4-(3-carboxyphenyl)pyridine-2,5-dicarboxylic acid 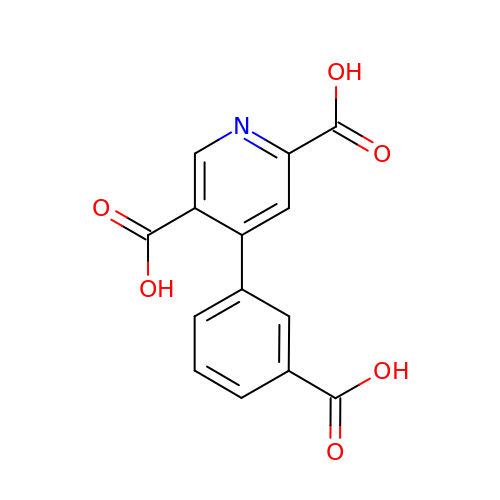| C14 H9 N O6 | NBVHLJGGHJLTGM-UHFFFAOYSA-N> LTESSTSKFVKINEKGFSDFNIHYNEAGNGETVIMLHGGGPGAGGWSNYYRNVGPFVDAGYRVILKDSPGFNKSDAVVMDEQRGLVNARAVKGLMDALDIDRAHLVGNAMGGATALNFALEYPDRIGKLILMGPGG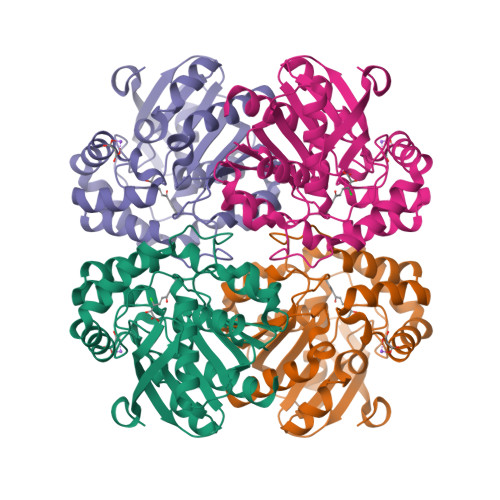LGPSMFAPMPMEGIKLLFKLYAEPSYETLKQMLQVFLYDQSLITEELLQGRWEAIQRQPEHLKNFLISAQKAPLSTWDVTARLGEIKAKTFITWGRDDRFVPLDHGLKLLWNIDDARLHVFSKCGHWAQWEHADEFNRLVIDFLRHA>[6x]MSDLNNAIQGILDDHVARGVVGVSLALCLPGEETSLYQSGYADKFNKMPMTGDHLFRIASCTKSFIATGLHLLVQDGTVDLDEPITRWFPDLPKAAQMPVRILLNHRSGLPDFETSMPMISDKSWTAQEIVDFSFRHGVQKEPWHGMEYSNTGYVLAGMIIAHETGKPYSDHLRSRIFAPLGMKDTWVGTHETFPIEREARGYMHAAADDENPQWDVSGAGDPVDGVWDSTEWFPLSGANAAGDMVST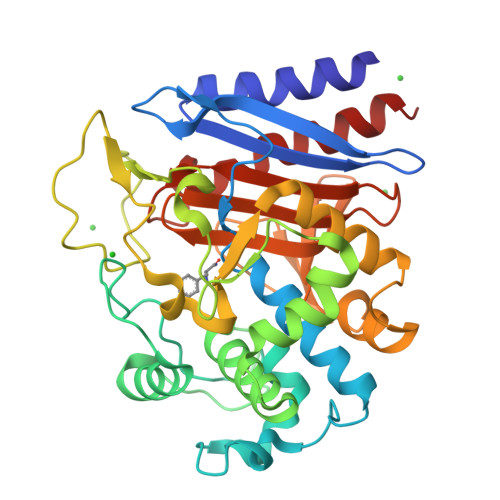PRDIVKFLNALFDGRILDQKRLWEMKDNIKPAFFPGSNTVANGHGLLLMRYGSSELKGHLGQIPGHTSIMGRDEETGAALMLIQNSGAGDFESFYLKGVNEPVDRVLEAIKNSRS>GHMTGTNTHSDVWIRQYRPAHPTAPQLICLPHAGGSATFYHPVAAALAPRCDVLAVQYPGRQDRRAEKPLEDIDELANQLFPVLRARVHQPVALFGHSMGATLAFELARRFESAGISLEALLVSARPAPSRQRTGGTV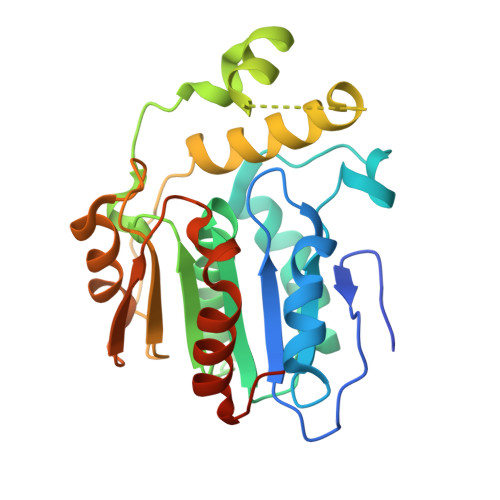HLLSDEELVAELRTLDGTAEQVFHDEELVRMALPAIRGDYRAAETYRYRPGPKLRCPIHALTGDDDPMVTPVEARAWSEHTDGPFTLDTFAGGHFYLLEHRDAILGIIAEHLRTCSRAPGDRSGLTRE[2x]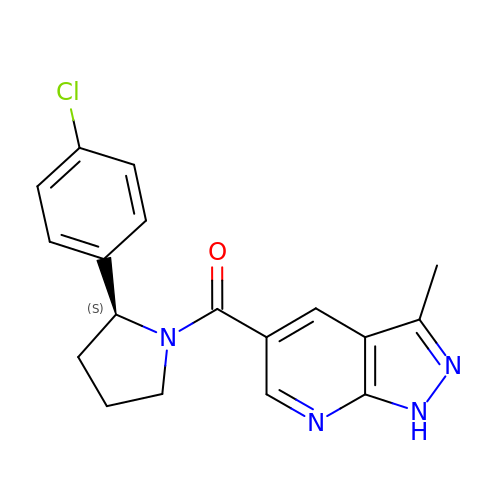[(2S)-2-(4-chlorophenyl)pyrrolidin-1-yl](3-methyl-1H-pyrazolo[3,4-b]pyridin-5-yl)methanone | C18 H17 Cl N4 O | ODRITQGYYWHQGM-INIZCTEOSA-N>[4x]TTIVSVRRNGHVVIAGDGQATLGNTVMKGNVKKVRRLYNDKVIAGFAGGTADAFTLFELFERKLEMHQGHLVKAAVELAKDWRTDRMLRKLEALLAVADETASLIITGNGDVVQPENDLIAIGSGGPYAQAAARALLENTELSAREIAEKALDIAGDICIYTNHFHTIEELSYK;>HHHHHHSEMTPREIVSELDKHIIGQDNAKRSVAIALRNRWRRMQLNEELRHEVTPKNILMIGPTGVGKTEIARRLAKLANAPFIKVEATKFTEVGYVGKEVDSIIRDLTDAAVKMVRVQAIEKNRYRAEELAEERILDVLIPPAKNNWGQTEQQQEPSAARQAFRKKLREGQLDDKEIEIDLAAAPMGVEIMAPPGMEEMTSQLQSMFQNLGGQKQKARKLKIKDAMKLLIEEEAAKLVNPEELKQDAIDAVEQHGIVFIDQIDKICKRGESSGPDVSREGVQRDLLPLVEGCTVSTKHGMVKTDHILFIASGAFQIAKPSDLIPELQGRLPIRVELQALTTSDFERILTEPNASITVQYKALMATEGVNIEFTDSGIKRIAEAAWQVNESTENIGARRLHTVLERLMEEISYDASDLSGQNITIDADYVSKHLDALVADEDLSRFIL[2x]

HslUV consists of one or two AAA+ HslU6 ring hexamers and the double-ring HslV12 peptidase (Rohrwild et al., 1997; Sousa et al., 2000; Wang et al., 2001). ATP-dependent proteolysis requires HslU6 to bind the degrons of target proteins in its axial channel and then unfold and translocate the substrate into the proteolytic chamber of HslV12. To reach the axial channel of the HslU hexamer, substrates must transit a funnel-like structure formed by segments of its intermediate (I) domain (Sousa et al., 2000; Wang et al., 2001). Here, we present evidence for a model in which HslU hexamers are autoinhibited at low temperatures by a trimeric I-domain plug that blocks the axial channel but melts at high temperatures to activate proteolysis.

We determined structures for three new crystal forms of E. coli HslU or HslUV by molecular replacement. Our new structures were similar to previous ones with the notable exception that a trimeric plug, formed by residues 183–206 of the I-domain, completely blocked the axial channel of the HslU ring. The plug consisted of amino acids from three of the six HslU subunits, each comprising an extended region (residues 183–188), a sharp turn (residues 189–191), and an α helix (residues 192–206). The three α helices that comprise the plug center packed together via hydrophobic contacts involving the side chains of Met192, Met195, Leu199, and Phe203. Additional hydrophobic packing contacts within the plug included Val184 and Ile186 from the extended region, which occupy peripheral grooves between plug helices, and Met202 from the helix. A Pro189-Pro190-Gly191 tripeptide formed a sharp turn between the extended region and α helix of the plug. The negatively charged side chains of Glu193 and Glu194 following this turn were also close to the positively charged side chains of Arg101 (94% conserved) and Lys293 (92% conserved) in the HslU axial channel, suggesting that favorable electrostatic interactions also stabilize the plugged conformation. Because protein substrates must access the axial channel of HslU to be engaged, unfolded, and translocated into the peptidase chamber of HslV, this plug would inhibit substrate degradation. We have identified a new conformation of the HslUV protease in which part of the I-domain forms a plug that blocks the axial channel of the AAA+ HslU ring and prevents productive substrate engagement and thus degradation. This plugged-channel inactive conformation is in dynamic equilibrium with an open-channel active conformation, with higher temperature and/or higher protein-substrate concentrations favoring the active conformation.> APVCVRP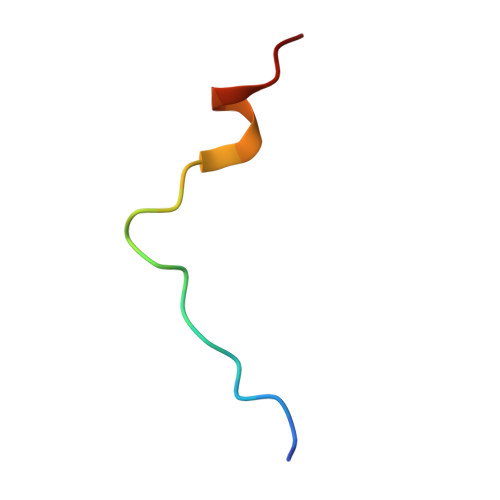TPKWQKGIGEFFAA> MGSVYDAWFSCASNQVAQVLLTLPYSFSQLGMMSGILFQLFYGLMGSWTAYLISVLYVEYRTRKEREKFDFRNHVIQWFEVLDGLLGKHWRNLGLIFNCTFLLFGSVIQLIACASNIYYINDKLDKRTWTYIFGACCATTVFIPSFHNYRIWSFLGLAMTTYTSWYLTIASLLHGQAEDVKHSGPTTMVLYFTGATNILYTFGGHAVTVEIMHAMWKPQKFKAIYLLAT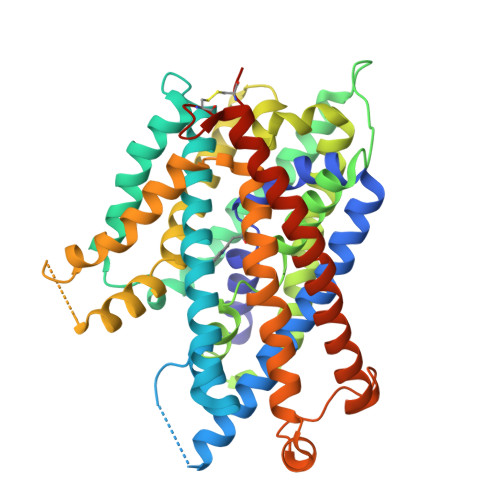IYVLTLTLPSASAVYWAFGDKLLTHSNALSLLPKTGFRDTAVILMLIHQFITFGFASTPLYFVWEKLIGVHETKSMFKRAMARLPVVVPIWFLAIIFPFFGPINSAVGSLLVSFTVYIIPALAHMLTFAPAPSRENAVERPPRVVGGWMGTYCINIFVVVWVFVVGFGFGGWASMVNFVRQIDTFGLFTKCYQCPPHKPGENLYFQ> MTQIIPALDLIDGEVVRLVKGDYEQKKVYKYNPLKKFKEYEKAGAKELHLVDLTGAKDPSKRQFALIEKLAKEVSVNLQVGGGIRSKEEVKALLDCGVKRVVIGSMA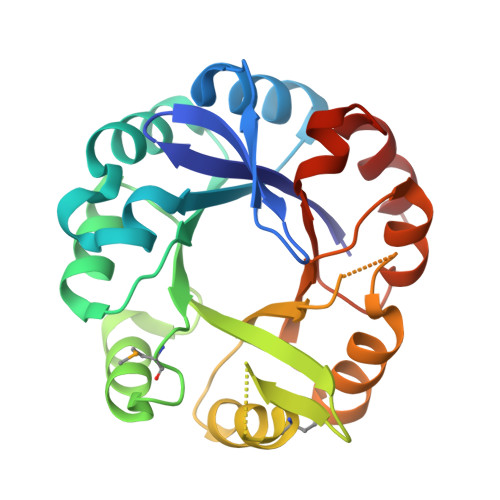IKDATLCLEILKEFGSEAIVLALDTILKEDYVVAVNAWQEASDKKLMEVLDFYSNKGLKHILCTDISKDGTMQGVNVRLYKLIHEIFPNICIQASGGVASLKDLENLKGICSGVIVGKALLDGVFSVEEGIRCLAN HD-PTP (His domain protein tyrosine phosphatase; PTPN23) is a non-receptor tumor suppressor phosphatase (Kok et al., 1997, Toyooka et al., 2000) that regulates several ubiquitin-dependent endosomal trafficking processes such as downregulation of EGFR and PDGFRβ signaling (Doyotte et al., 2008, Ma et al., 2015), recycling of Src (Chen et al., 2012, Lin et al., 2011), and degradation of α5β1 integrin (Kharitidi et al., 2015). HD-PTP drives the degradation of mitogenic receptors by coordinating their sorting into the multivesicular body (MVB) via specific recruitment of different endosomal sorting complexes required for transport (ESCRTs) (Ali et al., 2013, Stefani et al., 2011). HD-PTP has a multidomain organization that allows coordinated binding to several ESCRTs. The CC domain of HD-PTP is solely responsible for the interaction with UBAP1, and residue F678 in this domain is essential for binding (Stefani et al., 2011).

In order to define the molecular interactions, we determined the crystal structure of HD-PTPCC in complex with UBAP1C at 2.5 Å resolution. UBAP1C adopts a rather extended conformation and binds to the shaft, near the core of the three-strand coiled coil, between H4 and H7. Only residues 262–271 from UBAP1C were clearly identified in the electron density maps and the side chains of I263, L266, F268, P269, and L271 are in direct contact with HD-PTPCC. The binding interface in HD-PTPCC is defined by three hydrophobic pockets and the conserved FYX2L motif plays a critical role in the interaction. Pocket A is large and shallow and accommodates UBAP1C residues I263 and L266. Pocket B is deep and narrow and accommodates UBAP1C F268 and P269. Pocket C accommodates L271 and includes V504 (H4) and L682 (H7). In our HD-PTPCC-UBAP1C structure, the FY pair (F678, Y679) in HD-PTP forms stacking interactions with F268 in the FPXL motif of UBAP1C. Upon UBAP1C binding, E514, D667, and K671 side chains are displaced breaking the K671-D667 salt bridge and opening the A pocket. K671-Nζ then forms hydrogen bonds with the C=O groups of I263, K264, and L266 in UBAP1C.

> PMAAHEASSLYSEEKAKLLREMMAKIEDKNEVLDQFMDSMQLDPETVDNLDAYSHIPPQLMEKCAALSVRPDTVRNLVQSMQVLSGVFTDVEASLKDIRDLLEEDELLEQKFQEAVGQAGAISITSKAELAEVRREWAKYMEVHEKASFTNSELHRAMNLHVGNLRLLSGPLDQVRAALPTPALSPEDKAVLQNLKRILAKVQEMRDQRVSLEQQLRELIQKDDITASLVTTDHSEMKKLFEEQLKKYDQLKVYLEQNLAAQDRVLCALTEANVQYAAVRRVLSDLDQKWNSTLQTLVASYEAYEDLMKKSQEGRDFYADLESKVAALLERTQSTCQAREAARQQLLDRELK;> SNIKSLSFPKLDSDDSNQKT(3S,5Z,8S,9S,11E)-8,9,16-trihydroxy-14-methoxy-3-methyl-3,4,9,10-tetrahydro-1H-2-benzoxacyclotetradecine-1,7(8H)-dione 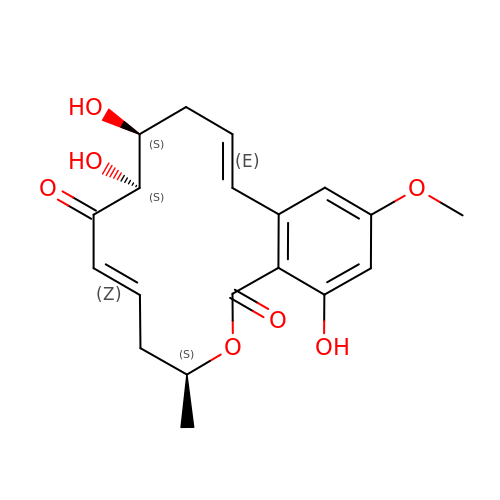| C19 H22 O7 | NEQZWEXWOFPKOT-BYRRXHGESA-N>[2x]KEMDPEKLKILEWIEGKERNIRALLSTMHTVLWAGETKW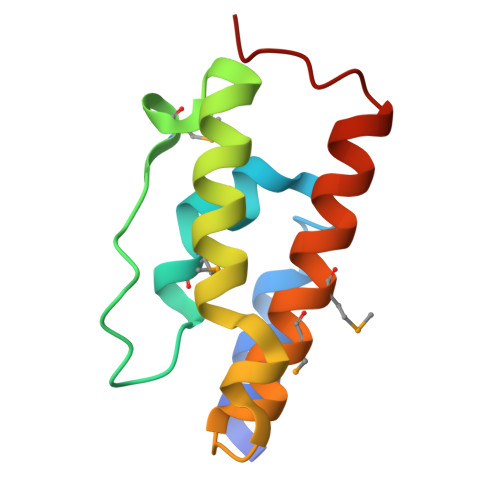KPVGMADLVTPEQVKKVYRKAVLVVHPDKATGQPYEQYAKMIFMELNDAWSEFENQGQKPLY>[5x]TVTYTNRVADARLGTFSQLLLQWKGSIYKLLYSEFLIFISLYFAISLVYRLILSESQRLMFEKLALYCNSYAELIPVSFVLGFYVSLVVSRWWAQYESIPWPDRIMNLVSCNVDGEDEYGRLLRRTLMRYSNLCSVLILRSVSTAVYKRFPSMEHVVRAGLMTPEEHKKFESLNSPHNKFWIPCVWFSNLAVKARNEGRIRDSVLLQGILNELNTLRSQCGRLYGYDWI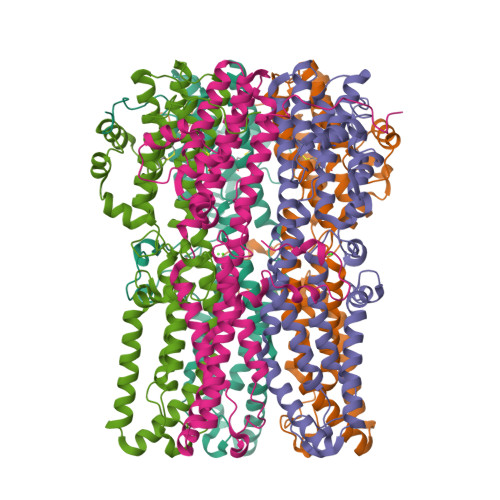SIPLVYTQVVTVAVYSFFLACLIGRQFLDPEKAYPGHELDLFVPVFTFLQFFFYAGWLKVAEQLINPFGEDDDDFETNWLIDRNLQVSLMAVDEMHQDLPILEKDLYWNEPDPQEGEEF> KSMQCKVILLDGSEYTCDVEKRSRGQVLFDKVCEHLNLLEKDYFGLTYRDAENQKNWLDPAKEIKKQVRSGAWHFSFNVKFYPPDPAQLSEDITRYYLCLQLRDDIVSGRLPCSFVTLALLGSYTVQSELGDYDPDECGSDYISEFRFAPNHTKELEDKVIELHKSHRGMTPAEAEMHFLENAKKLSMY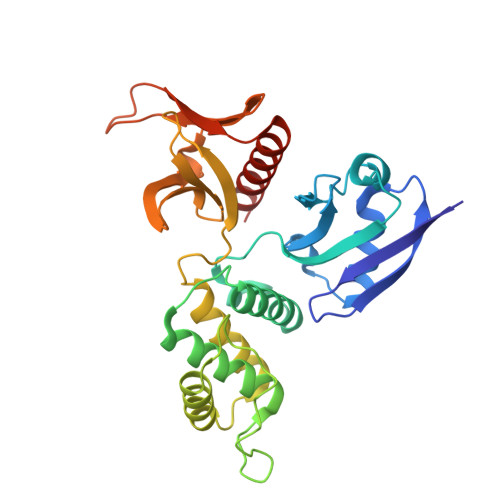GVDLHHAKDSEGVEIMLGVCASGLLIYRDRLRINRFAWPKVLKISYKRNNFYIKIRPGEFEQFESTIGFKLPNHRAAKRLWKVCVEHHTFFRLL> SFVKDFKPQALGDTN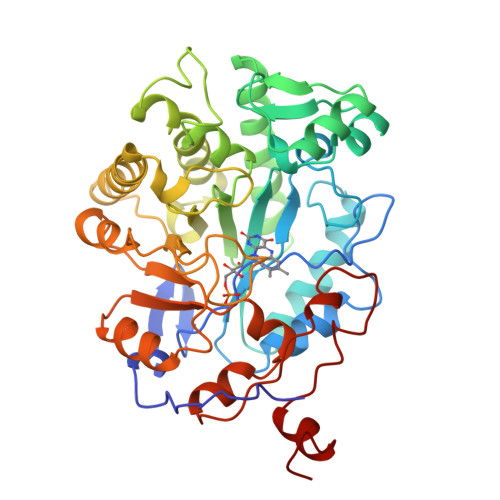LFKPIKIGNNELLHRAVIPPLTRMRALHPGNIPNRDWAVEYYTQRAQRPGTMIITEGAFISPQAGGYDNAPGVWSEEQMVEWTKIFNAIHEKKSFVWVQLWVLGWAAFPDNLARDGLRYDSASDNVFMDAEQEAKAKKANNPQHSLTKDEIKQYIKEYVQAAKNSIAAGADGVEINSANGYLLNQFLDPHSNTRTDEYGGSIENRARFTLEVVDALVEAIGHEKVGLRLSPYGVFNSMSGGAETGIVAQYAYVAGELEKRAKAGKRLAFVHLVEPRVTNPFLTEGEGEYEGGSNDFVYSIWKGPVIRAGNFALHPEVVREEVKDKRTLIGYGRFFISNPDLVDRLEKGLPLNKYDRDTFYQMSAHGYIDYPTYEEALKLGWDKS>[12x]TVTKTIETHTDNIETNMDENLRIPVTAEVGSGYFKMTDVSFDSDTLGKIKIRNGKSDAQMKEEDADLV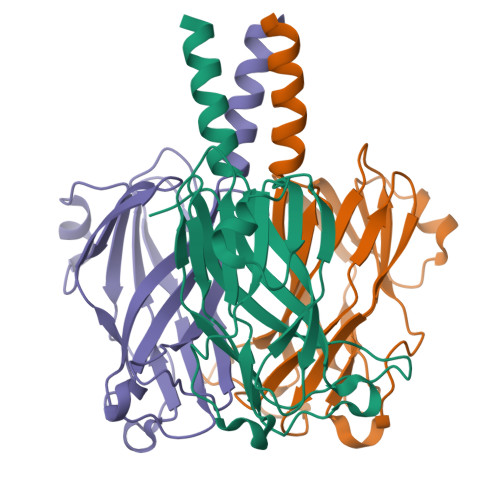ITPVEGRALEVTVGQNLTFEGTFKVWNNTSRKINITGMQMVPKINPSKAFVGSSNTSSFTPVSIDEDEVGTFVCGTTFGAPIAATAGGNLFDMYVHVTYSGT> GPMPGKSVVARVAEAYPEDVGKRVVRVDK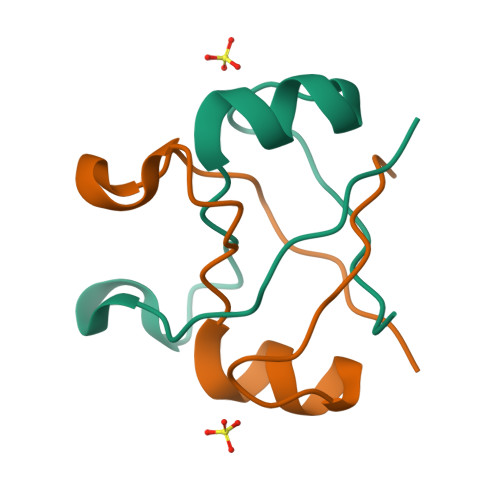YERAKVGVSVGDYVEVKKV> GPDETLSLLADPYRFISRQCQRLGA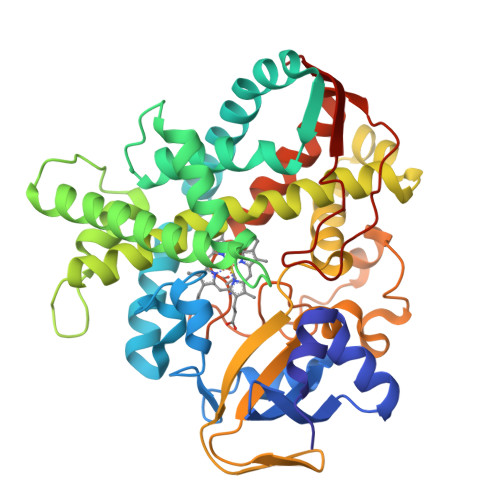NAFESRFLLKKTNCLKGAKAAEIFYDTTRFEREGAMPVAIQKTLLGQGGVQGLDGETHRHRKQMFMGLMTPERVRALAQLFEAEWRRAVPGWTRKGEIVFYDELHEPLTRAVCAWAGVPLPDDEAGNRAGELRALFDAAGSASPRHLWSRLARRRVDAWAKRIIEGIRAGSIGSGSGTAAYAIAWHRDRHDDLLSPHVAAVELVNVLRPTVEIAVYITFVAHALQTCSGIRAALVQQPDYAELFVQEVRRFYPFFPAVVARASQDFEWEGMAFPEGRQVVLDLYGSNHDAATWADPQEFRPERFRAWDEDSFNFIPQGGGDHYLGHRCPGEWIVLAIMKVAAHLLVNAMRYDVPDQDLSIDFARLPALPKSGFVMRNVHIGG> SMQFSKMHGLGNDFMVVDAVTQNVFFSPELIRRLADRHLGVGFDQLLVVEPPYDPELDFHYRIFNADGSEVAQCGNGARCFARFVRLKGLTNKRDIRVSTANGRMVLTVTDDDLVRVNMGEPNFEPSAVPFRANKAEKTYIMRAAEQTILCGVVSMGNPHCVIQVDDVDTAAVETLGPVLESHERFPERANIGFMQVVKREHIRLRVYERGAGETQACGSGACAAVAVGIQQGLLAEEVRVELPGGRLDIAWKGPGHPLYMTGPAVHVYDGFIHL;> SMIDDDGYRPNVGIVICNRQGQVMWARRFGQHSWQFPQGGINPGESAEQAMYRELFEEVGLSRKDVRILASTRNWLRYKLPKRLVRWDTKPVCIGQKQKWFLLQLVSGDAEI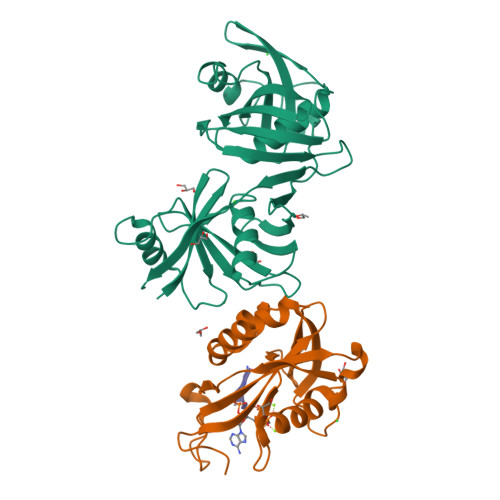NMQTSSTPEFDGWRWVSYWYPVRQVVSFKRDVYRRVMKEFASVVMSLA> AMKLISNDLRDGDKLPHRHVFNGMGYDGDNISPHLAWDDVPAGTKSFVVTCYDPDAPTGSGWWHWVVVNLPADTRVLPQGFGSGLVAMPDGVLQTRTDFGKTGYDGAAPPKGETHRYIFTVHALDIERIDVDEGAS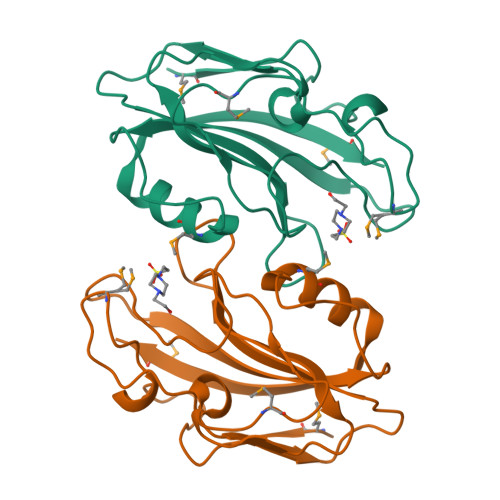GAMVGFNVHFHSLASASITAMFS Intracellular ADPR targets and activates the nonselective, calcium-permeable TRPM2 channel in the presence of Ca2+. Belonging to the transient receptor potential melastatin family (TRPM), TRPM2 shares a characteristic MHR1-4 domain, a transmembrane domain (TMD), and a coiled-coil domain with the other family members. It is unique due to owning a characteristic C-terminal NUDT9-H domain, which has been considered a classic binding site for ADPR and its derivatives, but the presence of the ADPR binding site has not been directly observed. In summary, our human TRPM2 structures defined two distinctive ADPR binding sites, one in the MHR1/2 domain and one in the NUDT9-H domain.

In the EDTA-hsTRPM2 structure, the NUDT9-H domain is clamped between cognate and adjacent MHR1/2 domains, forming both intra- and intersubunit interfaces, while only the intrasubunit interface exists in the EDTA-drTRPM2 structure. As a consequence, the NUDT9-H domain forms a compact structure interacting with the adjacent MHR1/2 domain in hsTRPM2, whereas it hangs freely in the drTRPM2 on the bottom of the protein. In the absence of ADPR, their interface is made of extensive interactions between the core region of NUDT9-H and MHR1. Accordingly, we call the interface between MHR1/2 and NUDT9-H a resting interface in the apo state and an activation interface in the ADPR-bound state. The EDTA-hsTRPM2 and the 8-Br-cADPR/Ca2+-hsTRPM2 structures were nearly identical, and they clearly represented an apo-resting state and an antagonist-bound inhibited closed state, respectively. By comparing the distances between the Cα of adjacent pore-restricting residues—N1049 and Q1053—with those in drTRPM2, all four showed an occluded pore, including the ADPR/Ca2+-hsTRPM2 structure. Lastly, the hsTRPM2 has a well-defined NUDT9-H domain that has two major interfaces with the rest of protein, one with the cognate MHR1/2 and the other with the adjacent MHR1/2 domain.

>[4x]GSGGRATMEPSALRKAGSEQEEGFEGLPRRVTDLGMVSNLRRSNSSLFKSWRLQCPFGNNDKQESLSSWIPENIKKKECVYFVESSKLSDAGKVVCQCGYTHEQHLEEATKPHTFQGTQWDPKKHVQEMPTDAFGDIVFTGLSQKVKKYVRVSQDTPSSVIYHLMTQHWGLDVPNLLISVTGGAKNFNMKPRLKSIFRRGLVKVAQTTGAWIITGGSHTGVMKQVGEAVRDFSLSSSYKEGELITIGVATWGTVHRREGLIHPTGSFPAEYILDEDGQGNLTCLDSNHSHFILVDDGTHGQYGVEIPLRTRLEKFISEQTKERGGVAIKIPIVCVVLEGGPGTLHTIDNATTNGTPCVVVEGSGRVADVIAQVANLPVSDITISLIQQKLSVFFQEMFETFTESRIVEWTKKIQDIVRRRQLLTVFREGKDGQQDVDVAILQALLKASRSQDHFGHENWDHQLKLAVAWNRVDIARSEIFMDEWQWKPSDLHPTMTAALISNKPEFVKLFLENGVQLKEFVTWDTLLYLYENLDPSCLFHSKLQKVLVEDPERPACAPAAPRLQMHHVAQVLRELLGDFTQPLYPRPRHNDRLRLLLPVPHVKLNVQGVSLRSLYKRSSGHVTFTMDPIRDLLIWAIVQNRRELAGIIWAQSQDCIAAALACSKILKELSKEEEDTDSSEEMLALAEEYEHRAIGVFTECYRKDEERAQKLLTRVSEAWGKTTCLQLALEAKDMKFVSHGGIQAFLTKVWWGQLSVDNGLWRVTLCMLAFPLLLTGLISFREKRLQDVGTPAARARAFFTAPVVVFHLNILSYFAFLCLFAYVLMVDFQPVPSWCECAIYLWLFSLVCEEMRQLFYDPDECGLMKKAALYFSDFWNKLDVGAILLFVAGLTCRLIPATLYPGRVILSLDFILFCLRLMHIFTISKTLGPKIIIVKRMMKDVFFFLFLLAVWVVSFGVAKQAILIHNERRVDWLFRGAVYHSYLTIFGQIPGYIDGVNFNPEHCSPNGTDPYKPKCPESDATQQRPAFPEWLTVLLLCLYLLFTNILLLNLLIAMFNYTFQQVQEHTDQIWKFQRHDLIEEYHGRPAAPPPFILLSHLQLFIKRVVLKTPAKRHKQLKNKLEKNEEAALLSWEIYLKENYLQNRQFQQKQRPEQKIEDISNKVDAMVDLLDLDPLKRSGSMEQRLASLEEQVAQTAQALHWIVRTLRASGFSSEADVPTLASQKAAEEPDAEPGGRKKTEEPGDSYHVNARHLLYPNCPVTRFPVPNEKVPWETEFLIYDPPFYTAERKDAAAMDPMGDTLEPLSTIQYNVVDGLRDRRSFHGPYTVQAGLPLNPMGRTGLRGRGSLSCFGPNHTLYPMVTRWRRNEDGAICRKSIKKMLEVLVVKLPLSEHWALPGGSREPGEMLPRKLKRILRQEHWPSFENLLKCGMEVYKGYMDDPRNTDNAWIETVAVSVHFQDQNDVELNRLNSNLHACDSGASIRWQVVDRRIPLYANHKTLLQKAAAEFGAHYFE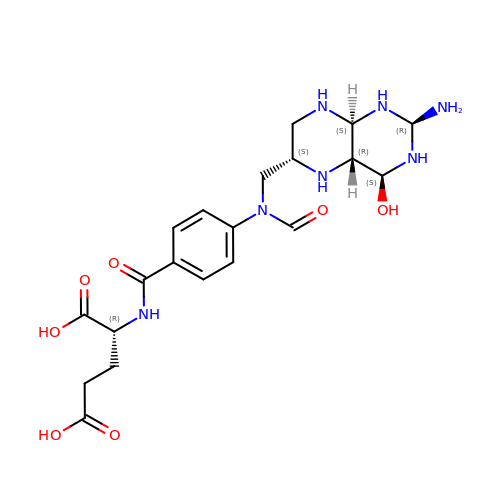N-({4-[{[(2R,4S,4aR,6S,8aS)-2-amino-4-hydroxydecahydropteridin-6-yl]methyl}(formyl)amino]phenyl}carbonyl)-D-glutamic acid | C20 H29 N7 O7 | VSNRWTPIADGZQS-GVIHMSOPSA-N> MRDTMEILRTENIVKYFGEFKALDGVSISVNKGDVTLIIGPNGSGKSTLINVITGFL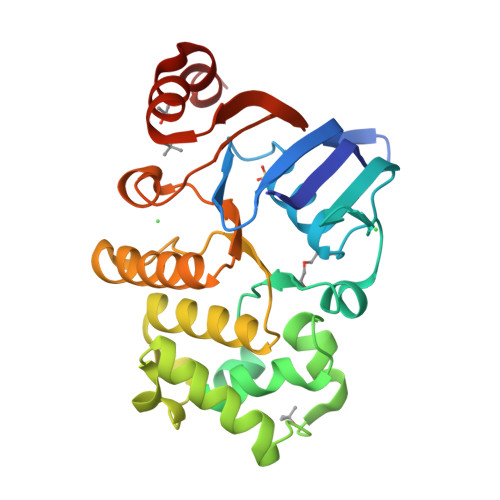KADEGRVYFENKDITNKEPAELYHYGIVRTFQTPQPLKEMTVLENLLIGEINPGESPLNSLFYKKWIPKEEEMVEKAFKILEFLKLSHLYDRKAGELSGGQMKLVEIGRALMTNPKMIVMDQPIAGVAPGLAHDIFNHVLELKAKGITFLIIEHRLDIVLNYIDHLYVMFNGQIIAEGRGEEEIKNVLSDPKVVEIYIGE In some pathogenic microbes, the response to oxidative stress is controlled by a SirTM/zinc-containing macrodomain (Zn-Macro) pair responsible for establishment and removal of the modification, respectively. Strikingly, however, the “catalytic loop” found in all other MacroD-type enzymes (also termed “loop 1”) is replaced with and extended loop containing the zinc-coordinating Cx(4)HxC motif, here termed the Zn-loop. To gain a closer understanding of the functional role of the 3α-bundle and coordinated Zn2+ ion, we solved structures from the three sub-branches of Zn-Macros namely from S. aureus (SauMacro), Methanobrevibacter oralis (MorMacro), and macrodomain-fused SirTM protein (Mfs1) from Fusarium oxysporum f.sp. cubense race 1 (Foc1Mfs1) in their apo form as well as of S. pyogenes (SpyMacro) and MorMacro bound to ADP-ribose (ADPr). In all structures, the Zn2+ ion is tetrahedrally coordinated with three metal-coordination residues within the Zn-loop, while the fourth coordination-contact is exchangeable and is provided by either ADPr, a water molecule, or a symmetry-related protomer within the crystal.

Interestingly, the major difference between the SpyMacro and MorMacro complex with ADPr is the form of the distal ribose. In SpyMacro, the ribose adopts a furanose ring with a 2′ endo pucker, while the distal ribose in MorMacro is in the linear form. The linear ribose isomer is usually disfavored in solution but has been observed in the Getah virus macrodomain. The open form is further stabilized via new contacts with Ala100 as well as the short 19SES21 stretch in a symmetry-related molecule. Surprisingly, neither MorMacro, which arises from a minimal operon containing only the Zn-Macro/SirTM pair, nor Zn-Macros derived from Msf1 fusion proteins could demodify SpyGcvH-L. In contrast, all Zn-Macros could demodify Glu-/Asp-ADP-ribosylated PARP1 E988Q.

>[2x]GPMNNDEQLEFLINYLLDERSESIDIPKTFSEKRNLLRSLMNMRHPSNISEEFLRIQDEFLSRETANKNLTSVEDISLSSGKIMLWQGDITTLSADAIVNAANSKLLGCFIPMHNCIDNIIHSASGLQLREECNRMIMLQGGDEDVGKAKITNAYNLPSKYVVHTVGPSIERGMRVSSDDVKKLERCYNSCLELASEYKLNSIAFCCISTGVFNFPQKKAAEIAIRTVKDFLNSNETSLNHIIFDVFTDKDYDIYKKLLFGN>[2x]MGAAILPDLGTEILIPVCAVIGIAFALFQWLLVSKVKLSAVRDASPNAAAKNGYNDYLIEEEEGINDHNVVVKCAEIQNAISEGATSFLFTEYKYVGIFMVAFAILIFLFLGSVEGFSTSPQACSYDKTKTCKPALATAIFSTVSFLLGGVTSLVSGFLGMKIATYANARTTLEARKGVGKAFITAFRSGAVMGFLLAANGLLVLYIAINLFKIYYGDDWGGLFAAITGYGLGGSSMALFGRVGGGIYTKAADVGADLVGK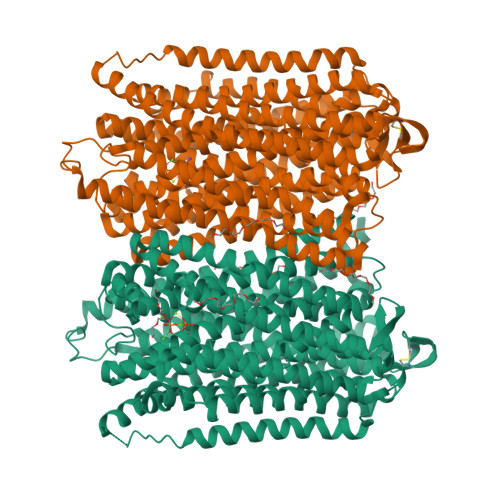VERNIPEDDPRNPAVIADNVGDNVGDIAGMGSDLFGSYAESSCAALVVASISSFGLNHELTAMLYPLIVSSVGILVCLLTTLFATDFFEIKAVKEIEPALKKQLVISTVLMTIGVAVVSFVALPTSFTIFNFGVQKDVKSWQLFLCVAVGLWAGLIIGFVTEYYTSNAYSPVQDVADSCRTGAATNVIFGLALGYKSVIIPIFAIAISIFVSFTFAAMYGIAVAALGMLSTIATGLAIDAYGPISDNAGGIAEMAGMSHRIRERTDALDAAGNTTAAIGKGFAIGSAALVSLALFGAFVSRASITTVDVLTPKVFIGLIVGAMLPYWFSAMTMKSVGSAALKMVEEVRRQFNTIPGLMEGTAKPDYATCVKISTDASIKEMIPPGALVMLTPLVVGILFGVETLSGVLAGSLVSGVQIAISASNTGGAWDNAKKYIEAGASEHARSLGPKGSDCHKAAVIGDTIGDPLKDTSGPSLNILIKLMAVESLVFAPFFATHGGLLFKIF> GPGTSTLSPGGGVTVFFHAIISLHFPFNPDLHKVFIRGGEEFGESKWDSNICELHYTRDLGHDRVLVEGIVCISKKHLDKYIPYKYVIYNGESFEYEFIYKHQQKKGEYVNRCLFIKSSLLGSGDWHQYYDIVYMKPHGRLQKVMNHITDGPRKDLVKGKQIAAALMLDSTFSILQTWDTINLNSFFTQFEQFCFVLQQPMIYEGQAQLWTDLQYREKEVKRYLWQHLKKHVVPLPDGKSTDFLPVDCPVRSKLKTGLIVLFVVEKIELLLEGSLDWLCHLLTSDASSPDEFHRDLSHILGIPQSWRLYLVNLCQRCMDTRTYTWLGALPVLHCCMELAPRHKDAWRQPEDTWAALEGLSFSPFREQMLDTSSLLQFMREKQHLLSIDEPLFRSWFSLLPLSHLVMYMENFIEHLGRFPAHILDCLSGIYYRLPGLEQVLNTQDVQDVQNVQNILEMLLRLLDTYRDKIPEEALSPSYLTVCLKLHEAICSSTKLLKFYELPALSAEIVCRMIRLLSLVDSAGQRDETGNNSVQTVFQGTLAATKRWLREVFTKNMLTSSGASFTYVKEIEVWRRLVEIQFPAEHGWKESLLGDMEWRLTKEEPLSQITAYCNSCWDTKGLEDSVAKTFEKCIIEAVSSACQSQTSILQGFSYSDLRKFGIVLSAVITKSWPRTADNFDDILKHLLTLADVKHVFRLCGTDEKILANVTEDAKRLIAVADSVLTKVVGDLLSGTILVGQLELIIKHKNQFLDIWQLREKSLSPQDEQCAVEEALDWRREELLLLKKEKRCVDSLLKMCGNVKHLIQVDFGVLAVRHSQDLSSKRLNDTVTVRLSTSSNSQRATHYHLSSQVQEMAGKIDLLRDSHIFQLFWREAAEPLSEPKEDQEAAELLSEPEEESERHILELEEVYDYLYQPSYRKFIKLHQDLKSGEVTLAEIDVIFKDFVNKYTDLDSELKIMCTVDHQDQRDWIKDRVEQIKEYHHLHQAVHAAKVILQVKESLGLNGDFSVLNTLLNFTDNFDDFRRETLDQINQELIQAKKLLQDISEARCKGLQALSLRKEFICWVREALGGINELKVFVDLASISAGENDIDVDRVACFHDAVQGYASLLFKLDPSVDFSAFMKHLKKLWKALDKDQYLPRKLCDSARNLEWLKTVNESHGSVERSSLTLATAINQRGIYVIQAPKGGQKISPDTVLHLILPESPGSHEESREYSLEEVKELLNKLMLMSGKKDRNNTEVERFSEVFCSVQRLSQAFIDLHSAGNMLFRTWIAMAYCSPKQGVSLQMDFGLDLVTELKEGGDVTELLAALCRQMEHFLDSWKRFVTQKRMEHFYLNFYTAEQLVYLSTELRKQPPSDAALTMLSFIKSNCTLRDVLRASVGCGSEAARYRMRRVMEELPLMLLSEFSLVDKLRIIMEQSMRCLPAFLPDCLDLETLGHCLAHLAGMGGSPVERCLPRGLQVGQPNLVVCGHSEVLPAALAVYMQTPSQPLPTYDEVLLCTPATTFEEVALLLRRCLTLGSLGHKVYSLLFADQLSYEVARQAEELFHNLCTQQHREDYQLVMVCDGDWEHCYLPSAFSQHKVFVTPQAPLEAIQAYLAGHYRVPKQTLSAAAVFNDRLCVGIVASERAGVGKSLYVKRLHDKMKMQLNVKNVPLKTIRLIDPQVDESRVLGALLPFLDAQYQKVPVLFHLDVTSSVQTGIWVFLFKLLILQYLMDINGKMWLRNPCHLYIVEILERRTSVPSRSSSALRTRVPQFSFLDIFPKVTCRPPKEVIDMELSALRSDTEPGMDLWEFCSETFQRPYQYLRRFNQNQDLDTFQYQEGSVEGTPEECLQHFLFHCGVINPSWSELRNFARFLNYQLRDCEASLFCNPSFIGDTLRGFKKFVVTFMIFMARDFATPSLHTSDQSPGKHMVTMDGVREEDLAPFSLRKRWESEPHPYVFFNDDHTTMTFIGFHLQPNINGSVDAISHLTGKVIKRDVMTRDLYQGLLLQRVPFNVDFDKLPRHKKLERLCLTLGIPQATDPDKTYELTTDNMLKILAIEMRFRCGIPVIIMGETGCGKTRLIKFLSDLRRGGTNADTIKLVKVHGGTTADMIYSRVREAENVAFANKDQHQLDTILFFDEANTTEAISCIKEVLCDHMVDGQPLAEDSGLHIIAACNPYRKHSEEMICRLESAGLGYRVSMEETADRLGSIPLRQLVYRVHALPPSLIPLVWDFGQLSDVAEKLYIQQIVQRLVESISLDENGTRVITEVLCASQGFMRKTEDECSFVSLRDVERCVKVFRWFHEHSAMLLAQLNAFLSKSSVSKNHTERDPVLWSLMLAIGVCYHASLEKKDSYRKAIARFFPKPYDDSRLLLDEITRAQDLFLDGVPLRKTIAKNLALKENVFMMVVCIELKIPLFLVGKPGSSKSLAKTIVADAMQGPAAYSDLFRSLKQVHLVSFQCSPHSTPQGIISTFRQCARFQQGKDLQQYVSVVVLDEVGLAEDSPKMPLKTLHPLLEDGCIEDDPAPHKKVGFVGISNWALDPAKMNRGIFVSRGSPNETELIESAKGICSSDILVQDRVQGYFASFAKAYETVCKRQDKEFFGLRDYYSLIKMVFAAAKASNRKPSPQDIAQAVLRNFSGKDDIQALDIFLANLPEAKCSEEVSPMQLIKQNIFGPSQKVPGGEQEDAESRYLLVLTKNYVALQILQQTFFEGDQQPEIIFGSGFPKDQEYTQLCRNINRVKICMETGKMVLLLNLQNLYESLYDALNQYYVHLGGQKYVDLGLGTHRVKCRVHPNFRLIVIEEKDVVYKHFPIPLINRLEKHYLDINTVLEKWQKSIVEELCAWVEKFINVKAHHFQKRHKYSPSDVFIGYHSDACASVVLQVIERQGPRALTEELHQKVSEEAKSILLNCATPDAVVRLSAYSLGGFAAEWLSQEYFHRQRHNSFADFLQAHLHTADLERHAIFTEITTFSRLLTSHDCEILESEVTGRAPKPTLLWLQQFDTEYSFLKEVRNCLTN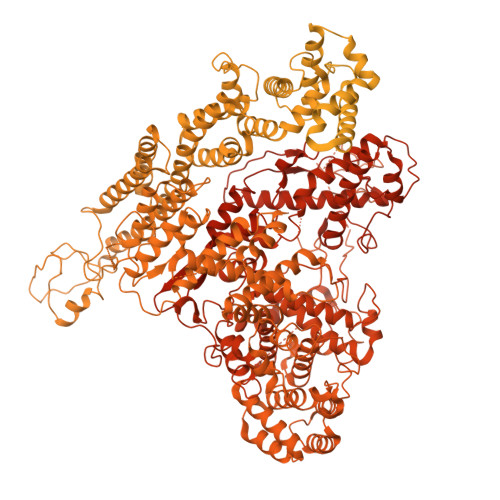TAKCKILIFQTDFEDGIRSAQLIASAKYSVINEINKIRENEDRIFVYFITKLSRVGRGTAYVGFHGGLWQSVHIDDLRRSTLMVSDVTRLQHVTISQLFAPGDLPELGLEHRAEDGHEEAMETEASTSGEVAEVAEEAMETESSEKVGKETSELGGSDVSILDTTRLLRSCVQSAVGMLRDQNESCTRNMRRVVLLLGLLNEDDACHASFLRVSKMRLSVFLKKQEESQFHPLEWLAREACNQDALQEAGTFRHTLWKRVQGAVTPLLASMISFIDRDGNLELLTRPDTPPWARDLWMFIFSDTMLLNIPLVMNNERHKGEMAYIVVQNHMNLSENASNNVPFSWKIKDYLEELWVQAQYITDAEGLPKKFVDIFQQTPLGRFLAQLHGEPQQELLQCYLKDFILLTMRVSTEEELKFLQMALWSCTRKLKAASEAPEEEVSLPWVHLAYQRFRSRLQNFSRILTIYPQVLHSLMEARWNHELAGCEMTLDAFAAMACTEMLTRNTLKPSPQAWLQLVKNLSMPLELICSDEHMQGSGSLAQAVIREVRAQWSRIFSTALFVEHVLLGTESRVPELQGLVTEHVFLLDKCLRENSDVKTHGPFEAVMRTLCECKETASKTLSRFGIQPCSICLGDAKDPVCLPCDHVHCLRCLRAWFASEQMICPYCLTALPDEFSPAVSQAHREAIEKHARFRQMCNSFFVDLVSTICFKDNAPPEKEVIESLLSLLFVQKGRLRDAAQRHCEHTKSLSPFNDVVDKTPVIRSVILKLLLKYSFHDVKDYIQEYLTLLKKKAFITEDKTELYMLFINCLEDSILEKTSAYSRNDELNHLEEEGRFLKAYSPASRGREPANEASVEYLQEVARIRLCLDRAADFLSEPEGGPEMAKEKQCYLQQVKQFCIRVENDWHRVYLVRKLSSQRGMEFVQGLSKPGRPHQWVFPKDVVKQQGLRQDHPGQMDRYLVYGDEYKALRDAVAKAVLECKPLGIKTALKACKTPQSQQSAYFLLTLFREVAILYRSHNASLHPTPEQCEAVSKFIGECKILSPPDISRFATSLVDNSVPLLRAGPSDSNLDGTVTEMAIHAAAVLLCGQNELLEPLKNLAFSPATMAHAFLPTMPEDLLAQARRWKGLERVHWYTCPNGHPCSVGECGRPMEQSICIDCHAPIGGIDHKPRDGFHLVKDKADRTQTGHVLGNPQRRDVVTCDRGLPPVVFLLIRLLTHLALLLGASQSSQALINIIKPPVRDPKGFLQQHILKDLEQLAKMLGHSADETIGVVHLVLRRLLQEQHQLSSRRLLNFDTELSTKEMRNNWEKEIAAVISPELEHLDKTLPTMNNLISQDKRISSNPVAKIIYGDPVTFLPHLPRKSVVHCSKIWSCRKRITVEYLQHIVEQKNGKERVPILWHFLQKEAELRLVKFLPEILALQRDLVKQFQNVQQVEYSSIRGFLSKHSSDGLRQLLHNRITVFLSTWNKLRRSLETNGEINLPKDYCSTDLDLDTEFEILLPRRRGLGLCATALVSYLIRLHNEIVYAVEKLSKENNSYSVDAAEVTELHVISYEVERDLTPLILSNCQYQVEEGRETVQEFDLEKIQRQIVSRFLQGKPRLSLKGIPTLVYRHDWNYEHLFMDIKNKMAQDSLPSSVISAISGQLQSYSDACEVLSVVEVTLGFLSTAGGDPNMQLNVYTQDILQMGDQTIHVLKALNRCQLKHTIALWQFLSAHKSEQLLRLHKEPFGEISSRYKADLSPENAKLLSTFLNQTGLDAFLLELHEMIILKLKNPQTQTEERFRPQWSLRDTLVSYMQTKESEILPEMASQFPEEILLASCVSVWKTAAVLKWNREMR>[2x]PSLLVLTFSPCVLLGWALLAGGTGGGGVGGGGGGAGIGGGRQEREALPPQKIEVLVLLPQDDSYLFSLTRVRPAIEYALRSVEGNGTGRRLLPPGTRFQVAYEDSDCGNRALFSLVDRVAAARGAKPDLILGPVCEYAAAPVARLASHWDLPMLSAGALAAGFQHKDSEYSHLTRVAPAYAKMGEMMLALFRHHHWSRAALVYSDDKLERNCYFTLE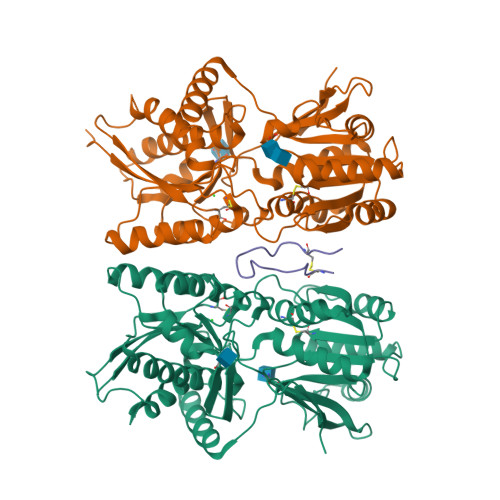GVHEVFQEEGLHTSIYSFDETKDLDLEDIVRNIQASERVVIMCASSDTIRSIMLVAHRHGMTSGDYAFFNIELFNSSSYGDGSWKRGDKHDFEAKQAYSSLQTVTLLRTVKPEFEKFSMEVKSSVEKQGLNMEDYVNMFVEGFHDAILLYVLALHEVLRAGYSKKDGGKIIQQTWNRTFEGIAGQVSIDANGDRYGDFSVIAMTDVEAGTQEVIGDYFGKEGRFEMRPNVKYPWGPLKLRIDENRIVEHTNSSPCKSSGGLE;> GCFGRKMDRISSSSGLGCKVL>AAGAAPVDISTLPRVKVDLVKPPFVHAHDQVAKTGPRVVEFTMTIEEKKLVIDREGTEIHAMTFNGSVPGPLMVVHENDYVELRLINPDTNTLLHNIDFHAATGALGGGALTQVNPGEETTLRFKATK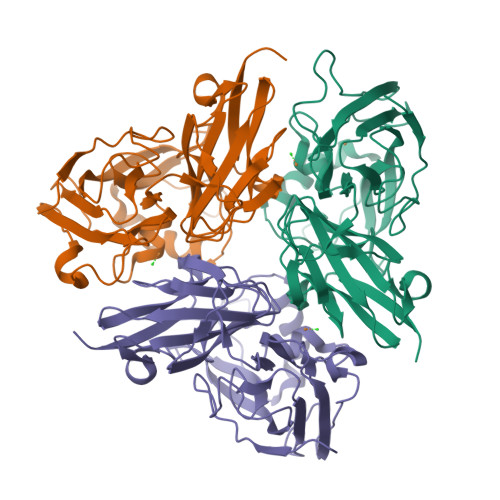PGVFVYHCAPEGMVPWHVTSGMNGAIMVLPRDGLKDEKGQPLTYDKIYYVGEQDFYVPKDEAGNYKKYETPGEAYEDAVKAMRTLTPTHIVFNGAVGALTGDHALTAAVGERVLVVHSQANRDTRPHLIGGHGDYVWATGKFRNPPDLDQETWLIPGGTAGAAFYTFRQPGVYAYVNHNLIEAFELGAAGHFKVTGEWNDD[6x]>[2x]GSAKDPSLPERIDTFTELFNYQLAEKSYDIRVLQSNYPTKLLSPDSMLPQTADYPLKDIQQLYQLANTCRGKLPLSPLITEPLVFTRAICKGTQLTPRWFSRSGLIHPGGGSYAARYVDKYP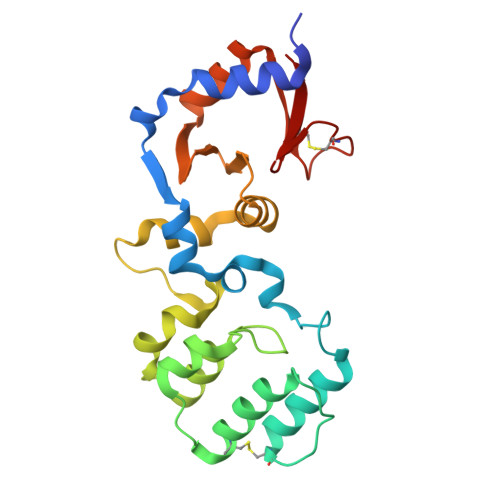ELQDKLAQYMHIKERKNVQGDELLASLKSMNDDAINALIAGASMFIEQNELWLRRGDHYFVFPKSVWQENVANAGLSFKLASQTKSCFVKRGNICWDVE> ARKREVRLMKNREAAR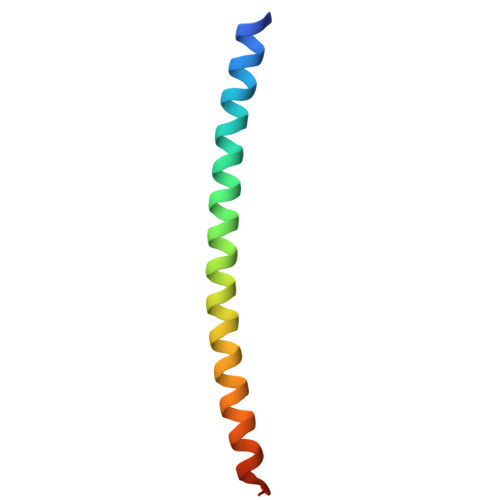ECRRKKKEYVKCLENRVAVLENQNKTLIEELKALKDLYCHKSD>[3x]TGTG;>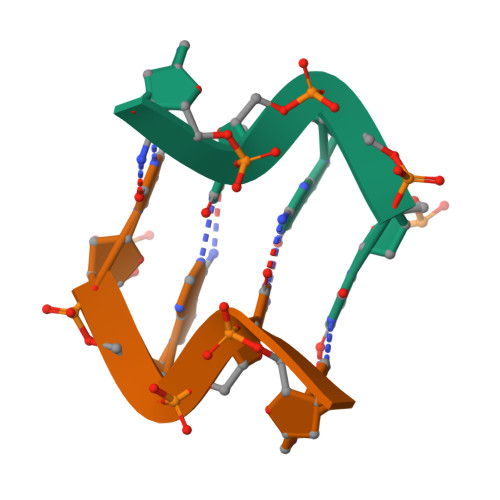[3x]CACA>MAHHHHHHMVHITLDPDTANPWLILSEDRRQVRLGDTQQSIPGNEERFDSYPMVLGAQHFHSGKHYWEVDVTGKEAWDLGVCRDSVRRKGHFLLSSKSGFWTIWLWNKQKYEAGTYPQTPLHLQVPPCQVGIFLDYEAGMVSFYNITDHGSLIYSFSECAFTGPLRPFFSPGFNDGGKNTAPLTLCPLNIGSQ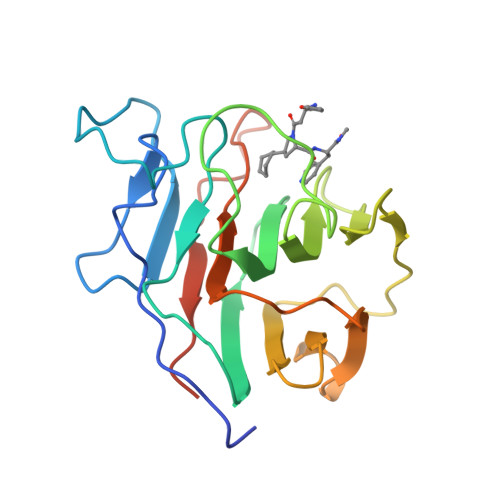GSTDY[2x]>[3x]MQDTDFFSWRRTMLLRFQRMETAEEVYHEIELQAQQLEYDYYSLCVRHPVPFTRPKVAFYTNYPEAWVSYYQAKNFLAIDPVLNPENFSQGHLMW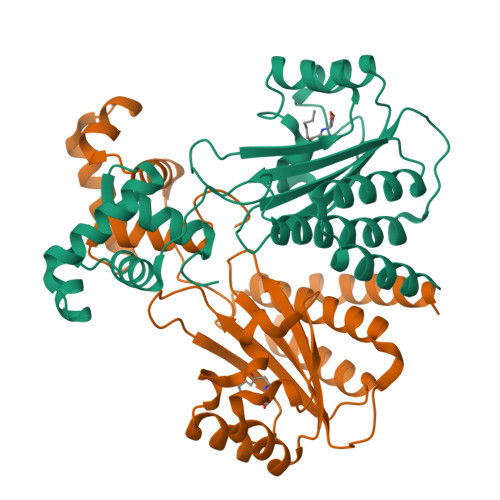NDDLFNEAQPLWEAARAHGLRRGVTQYLMLPNRALGFLSFSRCSAREIPILSDELQLKMQLLVRESLMALMRLNDEIVMTPEMNFSKREKEILRWTAEGKTSAEIAMILSISENTVNFHQKNMQKKINAPNKTQVACYAAATGLIHHHHHH> GPLGSPEFDCHLSDMLQQLHSVNASKPSERGLVRQEEAEDPACIPIFWVSKWVDYSDKYGLGYQLCDNSVGVLFNDSTRLILYNDGDSLQYIERDGTESYLTVSSHPNSLMKKIT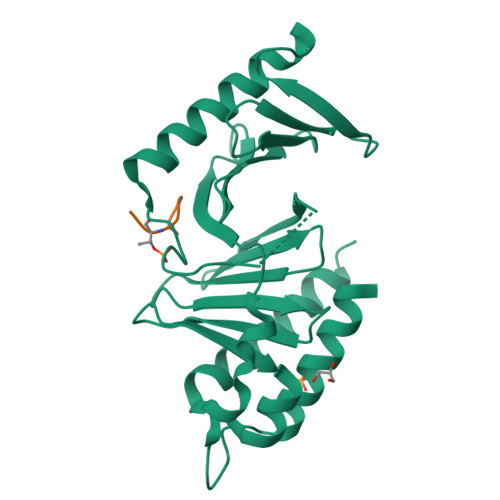LLKYFRNYMSEHLLKAGANITPREGDELARLPYLRTWFRTRSAIILHLSNGSVQINFFQDHTKLILCPLMAAVTYIDEKRDFRTYRLSLLEEYGCCKELASRLRYARTMVDKLLSSR;> XDPPLHSTAX>[2x]GMRALEQFANEFKVRRIKLGYTQTNVGEALAAVHGSEFSQTTICRFENLQLSFKNACKLKAILSKWLEEAEQV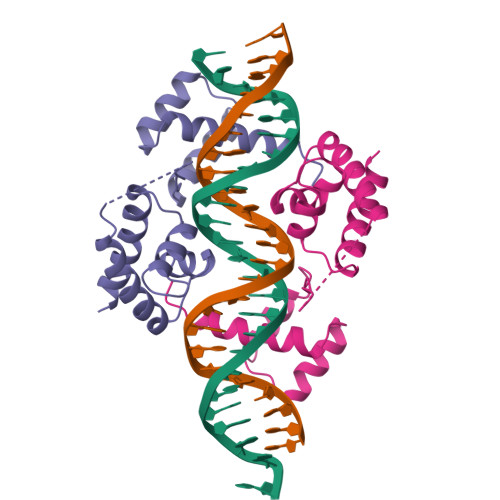GALYNEKVGANERKRKRRTTISIAAKDALERHFGEHSKPSSQEIMRMAEELNLEKEVVRVWFCNRRQREKRVK>VKGAPVFSQVVYQGNDRVYSENPLSPGEFYNPILQGCYPDPSITRKGDDYFLVCSSFAMFPGVPIFHSKDLVNWTQIGHVLDRTSQLKVHDTGISAGVYAPAIKYNPNNDTFYMITTQFAGGFGNIIVKSKDPFKGWSDPIKLNFDGIDPSIFFDDNGKAYVVHNDGPRRGEELYNGHRVIKIWEY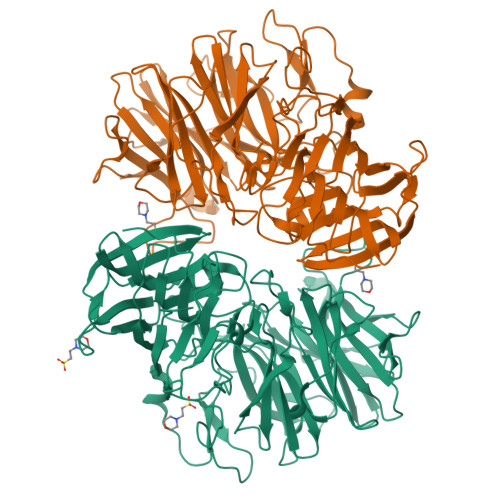DVENDQVIPGTDQVIVNGGVDLSKKPIWIEAPHIYKKDGRYYLMCAEGGTGGWHSEVIFVSDNPKGPFIPAPSNPDLSQRYLDHNRKNMVDWAGHADLVEGPDGKYYGVFLAIRPNEKGRVNIGRETFILPVDWSGEFPVFENGLIPMEPKLKTPAGVENKTGKDGYFPNGNFTFTENFTSPQLDYRWIGLRGPREEFISILKDGGLQVTPFPVNIKEVKPTSTLFYRQQHNNFSFTTTLNYTPKTEKDLAGITCVQSENFNYVFGLMKQDKDFHMVLAKTEKGNTRLLASAKVDMKNPIRLQVKGVGDNYDFSYSLDGNNFVLLGNTVSGDILSTNVAGGFTGCLIGLHATSANDIRV[2x]>ACDYTCGSNCYSSSDVSTAQAAGYKLHEDGETVGSNSYPHEFRNWNGFDFSVSSPYYEWPILSSGDVYSGG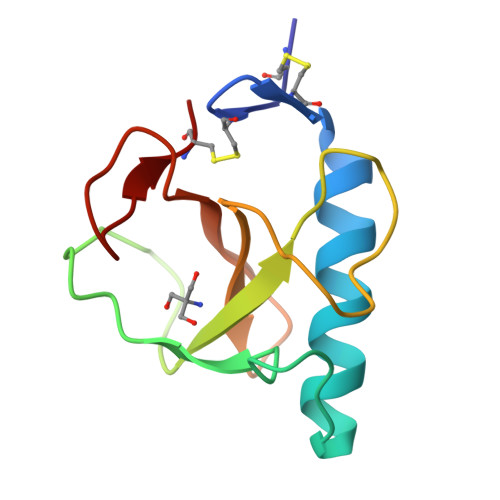SPGADRVVFNENNQLAGVITHTGASGNNFVECT[3x]The mammalian orthoreovirus (reovirus) σNS protein is required for formation of replication compartments that support viral genome replication and capsid assembly. In the case of mammalian orthoreoviruses, two nonstructural proteins, σNS and µNS, initiate VF formation, and σNS recruits viral RNAs into these compartments. Our crystallographic and biochemical studies reported here provide a mechanistic understanding of how σNS forms filamentous assemblies by linking dimeric units through domain-swapping interactions of the N-terminal arms and further how such a multimeric association is required for the RNA helix-destabilizing and RNA-annealing activities of σNS. An important finding from our studies is that mammalian orthoreovirus σNS has RNA helix-destabilizing and RNA-annealing activities without requiring a metal ion or ATP, which makes this protein an RNA chaperone.

We observed that the native σNS-R6A crystals, without Se-Met substitution, crystallized in the P41 space group instead of P65. Native σNS-R6A crystallized only in conditions with bile acid derivatives in contrast to Se-Met σNS-R6A, which crystallized without these additives. Structure determination of native σNS-R6A, using the Se-Met σNS-R6A structure as a molecular replacement model, showed that native σNS-R6A also forms an antiparallel dimer, with two bile acid moieties bound to each subunit in a groove located near the σNS C-terminus (sites 1 and 2). Binding of bile acid molecules is mediated by hydrophobic contacts with residues Thr 107, Glu 110, Leu 111, Ser 114, Gly 203, Leu 204, Tyr 240, Glu 242, Ala 245, and Glu 246. In contrast to the Se-Met σNS-R6A structure, the N-terminal arm is disordered and not observed in the native σNS-R6A structure. Instead of the distinct helical assembly in the structure of Se-Met σNS-R6A, native σNS-R6A dimers crystallized with bile acid show sheet-like packing. Further examination of the structure showed that one of the bile acid molecules occupies the same location in the core domain as the N-terminal arm required to form helical assemblies, suggesting that bile acid competes with the N-terminal arm to disrupt the helical assembly formation observed in the Se-Met σNS-R6A structure. First, the σNS crystal structure shows that the free N-terminal arm displaced by bile acid is disordered, as the electron density for this region is absent in the presence of bile acid. A fascinating finding from our study is that bile acid derivatives bind to the same site in σNS as the N-terminal arm and impede the RNA chaperone activity of σNS.

>MASSLRAAISKIKRDDVGQQVCPNYVMLRSSVTTKVVRNVVEYQIRTGGFFSCLAMLRPLQYAKRERLLGQRNLERISTRDILQTRDLHSLCMPTPDAPMSNHQASTMRELICSYFKVDHADGLKYIPMDERYSPSSLARLFTMGMAGLHITTEPSYKRVPIMHLAADLDCMTLALPYMITLDGDTVVPVAPTLSAEQLLDDGLKGLACMDISYGCEVDANSRPAGDQSMDSSRCINELYCEETAEAICVLKTCLVLNCMQFKLEMDDLAHNAAELDKIQMMIPFSERVFRMASSFATIDAQCFRFCVMMKDKNLKIDMRETTRLWTRSASDDSVATSSLSISLDRGRWVAADASDARLLVFPIRV[2x]> MEEGGSTGSAGSDSSTSGSGGAQQRELERMAEVLVTGEQLRLRLHEEKVIKDRRHHLKTY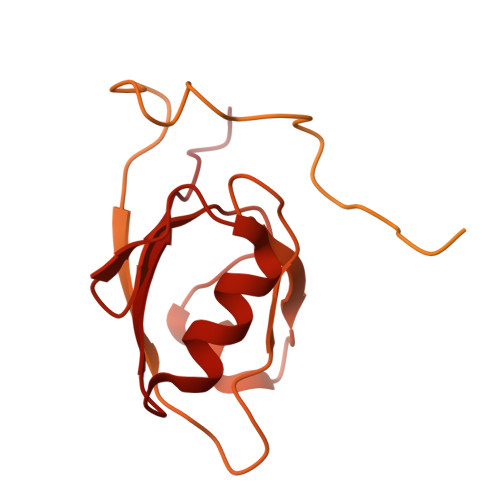PNCFVAKELIDWLIEHKEASDRETAIKLMQKLADRGIIHHVCDEHKEFKDVKLFYRFRKDDGTFPLDNEVKAFMRGQRLYEKLMSPENTLLQPREEEGVKYERTFMASEFLDWLVQEGEATTRKEAEQLCHRLMEHGIIQHVSSKHPFVDSNLLYQFRMNFRRRRRLMELLNEKSPSSQETHDSPFCLRKQSHDNRKSTSFMSVSPSKEIKIVSAVRRSSMSSCGSSGYFSSSPTLSSSPPVLCNPKSVLKRPVTSEELLTPGAPYARKTFTIVGDAVGWGFVVRGSKPCHIQAVDPSGPAAAAGMKVCQFVVSVNGLNVLHVDYRTVNNLILTGPRTIVMEVMEELEC>[4x]GUGAAAGUGUACCUA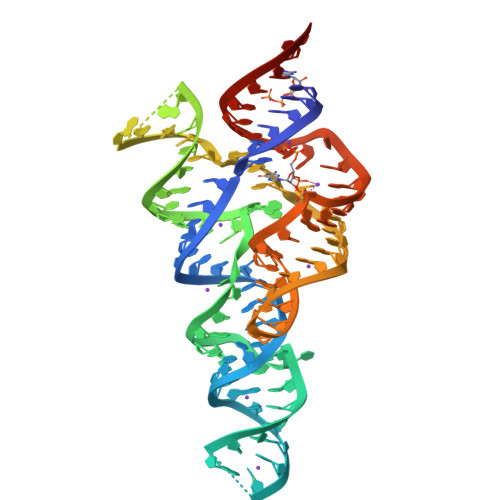GGGUUCCAGCCUAUUUGUAGGUGUUCGGACCGAGCGGUACAGGUAUAUUUUUAUAUACCACACCUUAGGGACAAAAGCCCGAGAGGAUAGGUUUCACUCGUA>SNAMQGGRFMGNKNLIITIEREYGSGGRIVGKKLAEELGIHFYDDDILKLASEKSAVGEQFFRLADEKAGNNLLYRLGGGRKIDLHSKPSPNDKLTSPENLFKFQSEVMRELAESEPCIFVGRAAGYVLDQDEDIERLIRIFVYTDKVKKVQRVMEVDCIDEERAKRRIKKIEKERKEYYKYFTGSEWHSMKNYDLPIN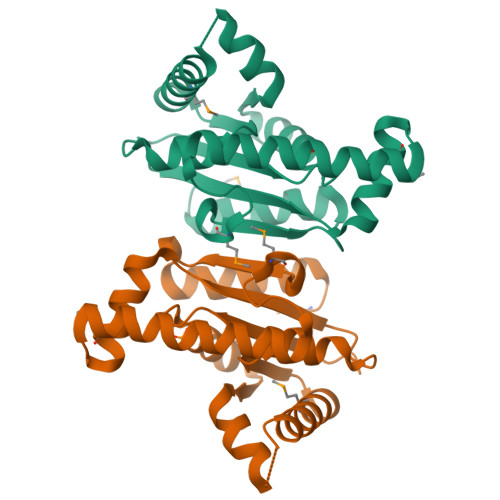TTKLTLEETAELIKAYIRLKGFMD[2x]>MAHHHHASGENLYFQGAMAAQSAVGSIETIGFPGILAAADAMVKAGRITIVGYIRAGSARFTLNIRGDVQEVKTAMAAGIDAINRTEGADVKT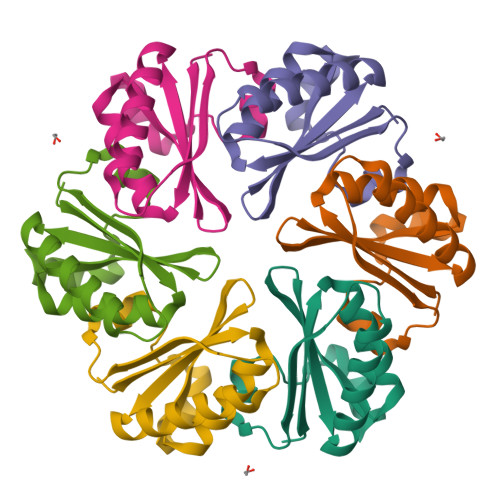WVIIPRPHENVVAVLPIDFSPEVEPFREAAEGLNRRA[2x]> TVQTSKNPQVDIAEDNAFFPSEYSLSQYTSPVSDLDGVDYPKPYRGKHKILVIAADERYLPTDNGKLFSTGNHPIETLLPL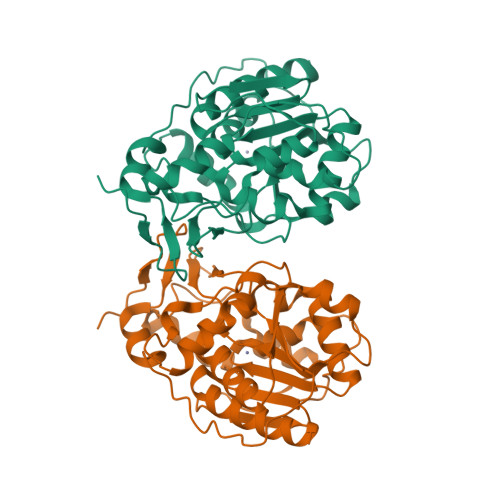YHLHAAGFEFEVATISGLMTKFEYWAMPHKDEKVMPFFEQHKSLFRNPKKLADVVASLNADSEYAAIFVPGGHGALIGLPESQDVAAALQWAIKNDRFVISLCHGPAAFLALRHGDNPLNGYSICAFPDAADKQTPEIGYMPGHLTWYFGEELKKMGMNIINDDITGRVHKDRKLLTGDSPFAANALGKLAAQEMLAAYAG> QDCYHGDGQSYRGTSSTTTTGKKCQSWSSMTPHRHQKTPENYPNAGLTMNYCRNPDADKGPWCFTTDPS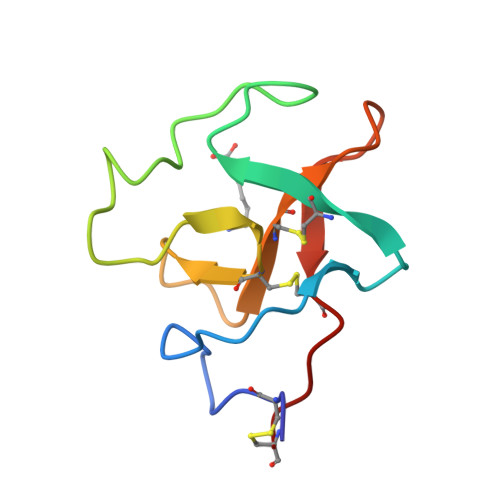VRWEYCNLKKC> SMIFSVQELSCGGKSMLSPTTRNMGASLSPQPDVSGELNTEALTRIVERLESEIIDGSWIHISYEETDLEMMPFLVAQANKKYPELNLKFVMSVHELVS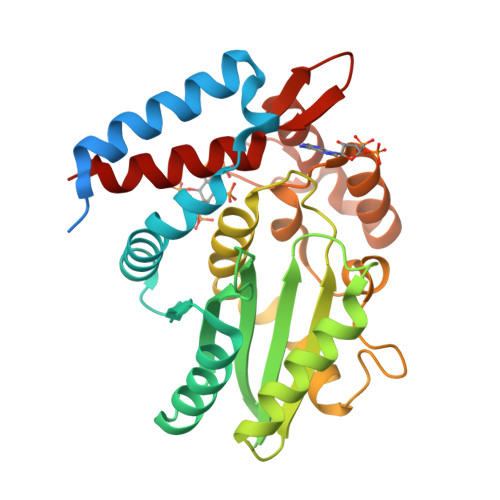SIKETRMEGVESARFLVNMGSSGIHISVVDFRVMDGKTSVILFEPAACSAFGPALALRTKAALEREQLPDCYFAMVELDIQRSSSECGIFSLALAKKLQLEFMNLVKIHEDNICERLCGEEPFLPSDKADRYLPVSFYKHTQGAQRLNEYVEANPAAGSSIVNKKNETLYERFDNNAVMLNDKKLSISAHKKRIAEYKSLLKP>[2x]GAFGGLPSLKSSFVLSEDTIPGTNETVKTLLPYGSVINYY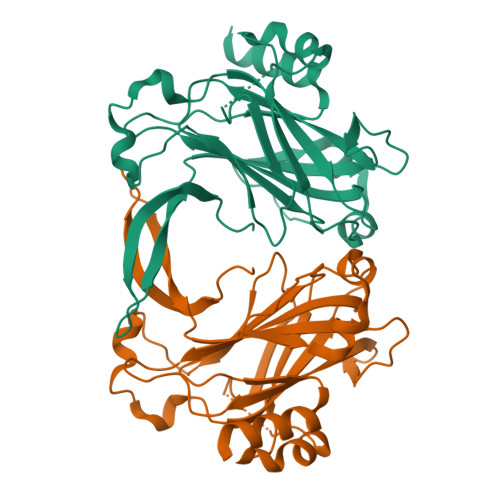GYVKPGQAPDGLVDGNKKAYYLYVWIPAVIAEMGVRMISPTGEIGEPGDGDLVSDAFKAATPEEKSMPHWFDTWIRVERMSAIMPDQIAKAAKAKPVQKLDDDDDGDDTYKEERHNKYNSLTRIKIPNPPKSFDDLKNIDTKKLLVRGLYRISFTTYKPGEVKGSFVASVGLLFPPGIPGVSPLIHSNPEELQKQAIAAEE>GFKQDIATIRGDLRTYAQDIFLAFLNKYPDEKRNFKNYVGKSDQELKSMAKFGDHTEKVFNLMMEVADRATDCVPLASDASTLVQMKQHSGLTTGNFEKLFVALVEYMRASGQSFDSQSWDRFGKNLVS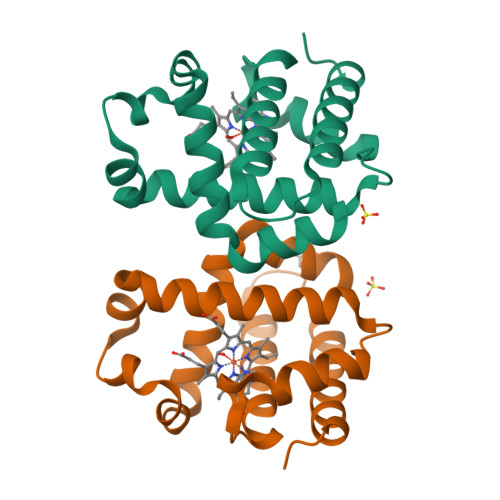ALSSAGMK[2x]>MKRIGVLTSGGDSPGMNAAIRSVVRKAIYHGVEVYGVYHGYAGLIAGNIKKLEVGDVGDIIHRGGTILYTARCPEFKTEEGQKKGIEQLKKHGIEGLVVIGGDGSYQGAKKLTEHGFPCVGVPGTIDNDIPGTDFTIGFDTALNTVIDAIDKIRDAATSHERTYVIEVMGRHAGDIALWSGLAGGAETILIPEADYDMNDVIARLKRGHERGKKHSIIIVAEGVGSGVDFGRQIQEATGFETRVTVLGHVQRGGSPTAFDRVLASRLGARAVELLLEGKGGRCVGI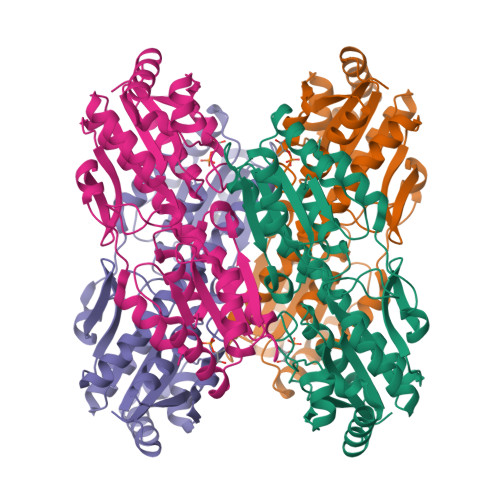QNNQLVDHDIAEALANKHTIDQRMYALSKELSI[4x]> DNENVVNEYSSELEKHQLYIDE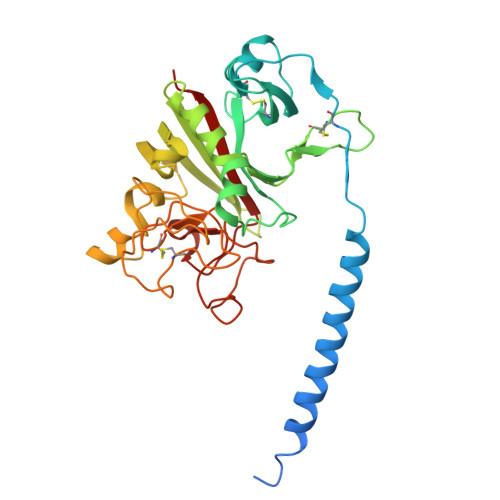TVNSNIPTNLRVLRSILENLRSKIQKLESDVSAQMEYCRTPCTVSCNIPVVSGKECEEIIRKGGETSEMYLIQPDSSVKPYRVYCDMNTENGGWTVIQNRQDGSVDFGRKWDPYKQGFGNVATNTDGKNYCGLPGEYWLGNDKISQLTRMGPTELLIEMEDWKGDKVKAHYGGFTVQNEANKYQISVNKYRGTAGNALMDGASQLMGENRTMTIHNGMFFSTYDRDNDGWLTSDPRKQCSKEDGGGWWYNRCHAANPNGRYYWGGQYTWDMAKHGTDDGVVWMNWKGSWYSMRKMSMKIRPFFPQQ> GPTI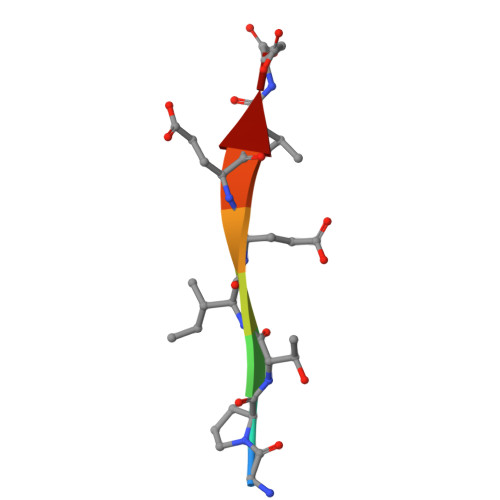EEVD> MNDIIINKIATIKRCIKRIQQVYGDGSQFKQDFTLQDSVILNLQRCCEACIDIANHINRQQQLGIPQSSRDSFTLLAQNNLITQPLSDNLKKMVGLRNIAVHDYQELNLDIVVHVVQHHLEDFEQFIDVIKAEHHHHH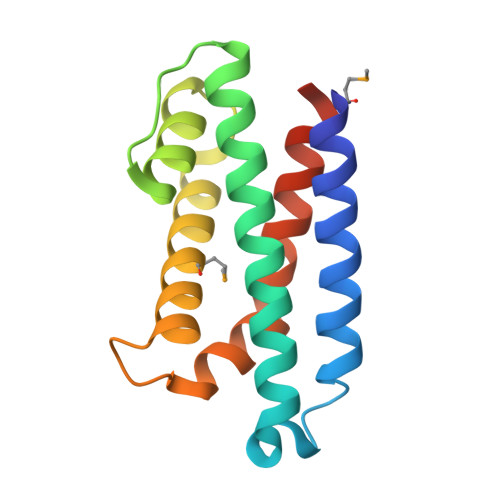H>[16x]MSQLAHNL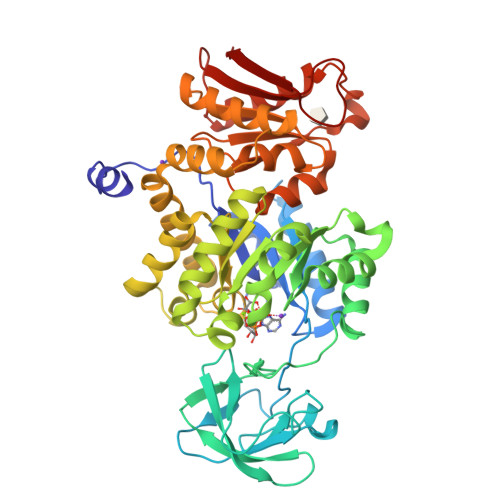TLSIFDPVANYRAARIICTIGPSTQSVEALKGLIQSGMSVARMNFSHGSHEYHQTTINNVRQAAAELGVNIAIALDTKGPEIRTGQFVGGDAVMERGATCYVTTDPAFADKGTKDKFYIDYQNLSKVVRPGNYIYIDDGILILQVQSHEDEQTLECTVTNSHTISDRRGVNLPGCDVDLPAVSAKDRVDLQFGVEQGVDMIFASFIRSAEQVGDVRKALGPKGRDIMIICKIENHQGVQNIDSIIEESDGIMVARGDLGVEIPAEKVVVAQKILISKCNVAGKPVICATQMLESMTYNPRPTRAEVSDVANAVFNGADCVMLSGETAKGKYPNEVVQYMARICLEAQSALNEYVFFNSIKKLQHIPMSADEAVCSSAVNSVYETKAKAMVVLSNTGRSARLVAKYRPNCPIVCVTTRLQTCRQLNITQGVESVFFDADKLGHDEGKEHRVAAGVEFAKSKGYVQTGDYCVVIHADHKVKGYANQTRILLVE The pseudokinase STRAD activates the LKB1 tumour suppressor by forming a heterotrimeric complex with LKB1 and the scaffolding protein MO25. In humans, there are two closely related isoforms of STRAD (STRADα and STRADβ) and MO25 (MO25α and MO25β) that similarly interact with and activate LKB1. Unlike the majority of kinases that require phosphorylation of their T-loop, LKB1 is activated through direct interaction with STRADα/β isoforms. MO25α is composed of seven structurally similar α-helical repeats (named R0–R6) that form a horseshoe-shaped molecule with a concave and a convex surface.

Here, we report the structure of STRADα as part of the STRADα/MO25α heterodimer. With the help of chemical lysine methylation, diffraction of these crystals (retaining the same space group and unit cell dimensions) improved to 2.35 Å. The structure of STRADα exhibits the classical bilobal protein kinase fold, with the N-terminal lobe (residues 59–152) organized around a central β-sheet, and a C-terminal lobe (residues 153–401) that is largely α-helical. A well-resolved molecule of ATP was observed in the cleft between the small and large lobes of the pseudokinase. Met83 replaces one of the conserved Gly residues in the glycine-rich loop, Arg100 substitutes the catalytic Lys residue in the VAIK motif, Ser195 replaces the Asp residue in the HRD motif, His200 substitutes for the conserved Asn in subdomain-VIb, and the entire DFG motif is replaced by GLR (residues 213–215). Consistent with the lack of the DFG motif in STRADα, no Mg2+ ions were observed in the STRADα-ATP complex, despite 1 mM MgCl2 being present in the crystallization mother liquor. The β-phosphate is tethered through interactions with Arg215 from the GLR (DFG) motif, and His200 (subdomain-VIb), basic residues that may substitute for one of the positively charged Mg2+ ions. Although the activation loop of STRADα (residues 212–245) is not phosphorylated, it is well ordered, a feature normally observed only in structures of activated protein kinases that are phosphorylated on their activation loop. Strikingly, the crystal structure of the STRADα/MO25α complex reveals that, in addition to the interaction through the WEF motif, a major additional binding interface involves the STRADα N-terminal kinase lobe and the MO25α concave surface. The αC-helix of STRADα runs along the concave surface of MO25α facing the H3 helixes of the MO25α repeats R4, R3, and R2 (termed the “αC site” here).

> MPFPFGKSHKSPADIVKNLKESMAVLEKQDISDKKAEKATEEVSKNLVAMKEILYGTNEKEPQTEAVAQLAQELYNSGLLSTLVADLQLIDFEGKKDVAQIFNNILRRQIGTRTPTVEYICTQQNILFMLLKGYESPEIALNCGIMLRECIRHEPLAKIILWSEQFYDFFRYVEMSTFDIASDAFATFKDLLTRHKLLSAEFLEQHYDRFFSEYEKLLHSENYVTKRQSLKLLGELLLDRHNFTIMTKYISKPENLKLMMNLLRDKSRNIQFEAFHVFKVFVANPNKTQPILDILLKNQAKLIEFLSKFQNDRTEDEQFNDEKTYLVKQIRDLKRPAQQEA;> MAHHHHHHMENLYFQGMSSFLPEGGCYELLTVIGKGFEDLMTVNLARYKPTGEYVTVRRINLEACSNEMVTFLQGELHVSKLFNHPNIVPYRATFIADNELWVVTSFMAYGSAKDLICTHFMDGMNELAIAYILQGVLKALDYIHHMGYVHRSVKASHILISVDGKVYLSGLRSNLSMISHGQRQRVVHDFPKYSVKVLPWLSPEVLQQNLQGYDAKSDIYSVGITACELANGHVPFKDMPATQMLLEKLNGTVPCLLDTSTIPAEELTMSPSRSVANSGLSDSLTTSTPRPSNGDSPSHPYHRTFSPHFHHFVEQCLQRNPDARPSASTLLNHSFFKQIKRRASEALPELLRPVTPITNFEGSQSQDHSGIFGLVTNLEELEVDDWEF(3S)-5-[(2-CHLORO-6-FLUOROBENZYL)SULFANYL]-3-{[N-({2-ETHOXY-5-[(1E)-3-METHOXY-3-OXOPROP-1-ENYL]PHENYL}ACETYL)-D-VALYL]AMINO}-4-OXOPENTANOIC 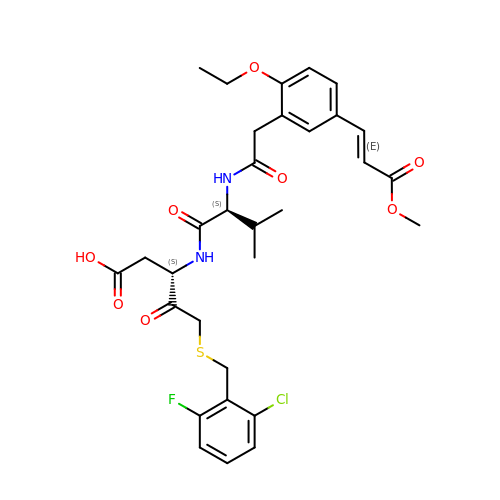ACID | C31 H36 Cl F N2 O8 S | BBHZJDWNUYJWFP-FSJABKHUSA-N> GHMGRSSRKDEILQAALACFSEHGVDATTIEMIRDRSGASIGSLYHHFG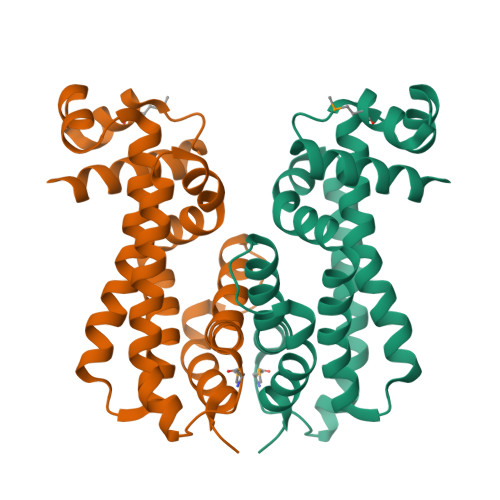NKERIHGELYLAGIGQYAALLEAGFARARSAEETVRLLVTSYIDWVVANPDWARFILHSRGRVEAGELGERLRADNQAHFARIHAALAGYRAEGLFREMPDDCFASVVIGPAHDLARQWLAGRTRVALADCRELLAQVAWDSVRAAGS>[12x]MVDVKKLLGKRDNSKLYEEIRKETKPKLDVNRLCRMRNDAKSDLDMWRSILQTAYHYAMPDYNPFENYGLAGFLTPGQQYNADIYDLTLPIAHKRLADKMLMNMVPQGQQWVKFTPGDEFGEPGTPLYQRALDATQRMTDHFFKIIDRSNFYLAVGESLQDVLISTGIIAINEGNRKRPVRYEAVPPAQVMFQGDAEGQVDAIFRDWYQVRIENIKSMWPKAEVAKLNKKPEDKVDIWECAWIDYEAPEKERYQYVVMTSSKDVLLEQSNSSWPWVVYRMRRLTGEIRGRGPSLSAYPTAATINQALEDELVAAAFQANPMYMAASDSAFNQQTFTPRPGSIVPVQMVQGEWPIKPFEQSGNIQFNALLVNDFRQQINELLYAFPLGAVNSPTRTATEAEIRYTENLESFSAMVPRLQNEFFIPVIQRTLWVINKVLPETFANIPDDIRNKMISVDGQILGLSFDTPLMTAKGQVKTAALLGFYQAAASLLGPEAATASLDPVEVLTNLADNQGIDVRNIKTREELEQLLQAAGQIAQQEAAQQGVIIGSEQPQ;>MIELTSAPTTKIEIISAAISMVGKQQTVNTIDGGGALAIDAEKLYDTLVSAELGSNRWRFAQAFQQISIITTLNPTFDGWLYECQIPADCIMVQYLYPNIQYIVFGDKILTKSNQTFTLIYSRNVPVSKWPPPFSLYIVYHLASMLGISVTNSDRMLARISQGMEMWESRALFADAQSSVTLPFRHNPYVDVRYRYKTRGY[12x];>MSNIKINDVFQRIQYAASAGQTQFTIPFPFF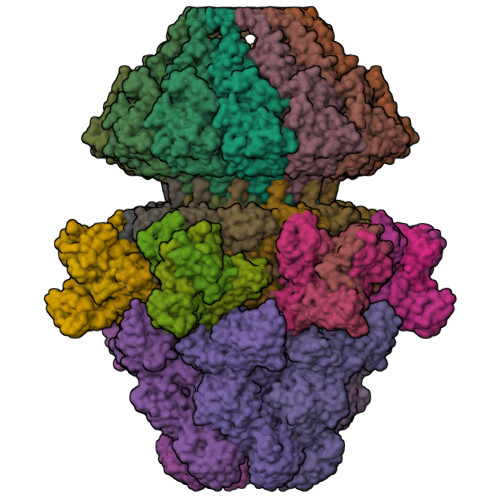DNEYVLVWQNGVQLVMGGAPGQYGISGAGSPSGGLITLVTPAALNDIITIQGDMPIDRTSIYSATISNLTGSDLNGDFNREVVMMKQIQTTQALLQLQYAPWLEVSQDPDVTKDRYLPLLGSGQVWRMNDSGTGIEAYTIDETPAPSSSPFIIYQADATLSNAQNLGALTSGILKQTVGGGSSTLSIAQNAVDYWAPGDELTRSQAPVSPDDVVNKAYADSIASGFTFINPVNAASTANFNSTYNNGSSGVGATLTATSNGAFSLDGQAGVLNKSYLMKDQTNTFENGIYILTQVGDGSTPAILTRATYFDQPSEIQPGDLVPVLAGTVNNGTLWLQTDTVSAVGTDPITFIAFLPAFSNIVTISGNQTITGDKTFTGTTTLDNFIFVGSNIQHLGDTGNQIIFGTATQINTINNNTISDLSSSGLRLGAANARVSTILDEDDMASDSATALATQQSIKAYVDNFRAAGAILQTVSTNMTNTFSASLAAGSGFSDVTGFNVSITPSATANKVFIKVDMLLASDTVDIVVVVRLKRNGTPIDIGNAAGSRIQITTGSTNAKALDGLQAVSFSFLDSPATTSAITYQVDIGQRTSGSAVGIVVNRSGADVDSSSYTRGASTITAQEIKG[18x];>MPIRSISNTFNRGELDPTLFARDDLDIYDKGARKLRNMIALWTGAARIAPGTIYIDMMVDRENGNAVIQDPLMVKGFDFTYDADAEITYTIIIRKSGTNIAFDIYYADTLQTTVTSTAYLATQIQDIHVAAAHDRVLILHENVQIRQLKRGASHSSWSLTTFNPRVYPTYDFSVIGEAINYQSFTFTLSATTGSITITSSSAVFTHNHVGGLFRSLGGTARITAVASTTSASATVLDNFTGTSCAGNLSSLAEKLWNSDTTTAPVSANRGWPARGVFYLNRLILGRSLAVKNLVNLSTAGVYDNFDDADLDGLVAFSVTFNGKGEQSVQSIVADDSILFTTANKLFAQSPLVESPITINNVYFAPQSQSPATSIEAASIDNQTLFVSSDRTKVMQAMYSTADGKYITLPATMLSNSIVDYINSNGTWEPAGISTRLYLATQDNGTMLLYSTLQTQNVAGWSLRTTTGKFRQVIGEGRQSHVIVEREINIGASFEQTLDYAYLSDPTFKARYDVTEFFASSPMTSAIGVLENQNDYILIGNQAPFTALDIDFNLVASSDCQLQFEYLDGNGFWDVFTPTDNTSGFTVDGTITWTFDDVLNWAPYQVNAIENQYWIRIKRLAETVNTAPVIGQVLINTGNRIYLERQSFDEYMDSTQIVTSDSNGLVTGLTHLAGQQVYAITEDGATIGSSFVDASGETSVKNVNTTLTVGMQYKPELIPMPLYAPTQMGDSLYAEKYVQDLYVDYVDSLYLQAGFRPQLTDIPNMHLGNYTLGQSVPPQTGIYRICPRGDWEPRQEFVITQSQPGPMTIIGVGYNVEVA[6x]>[2x]MKIAVIGQSLFGQEVYKELKNEGHMIVGVFTIPDKDGKVDPLAIEAEKDGVPVFKFPRWRLKGKAITEVVDQYKAVGAELNVLPFCSQFIPMEVIDHPKHGSIIYHPSLLPRHRGASAINWTLIHGDKKGGFTVFWADDGLDTGPILLQRECDVEPNDNVNSIYKRFLFPEGVKGMVEAVRLIATGKAPRIKQPEEGATYECIQKKE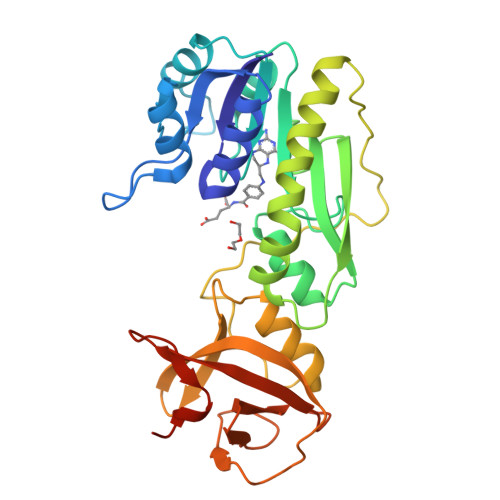NSKIDWNQPAEAIHNWIRGNDRVPGAWAEIDGKSVSFYGSTLLENDHFSSNGQPLEIPGASRAALVTKNGLVLFGNDGKMLLVKNLQFEDGKMIPGSQYFKAGVEHHHHHH>MANPTLFVSYDQNGKKLSFANWISVLSPQDTPFVSMTGKESINQTIFSWQTDALASVDGNNAHVEGSRAEDGEMKPTVIKSNVTQILRKVVRVSDTANTTANYGRGRELMYQLEKKGKEIKRDLEKILLSGQARTDVLADQYLTNSAADPAVAGLNDTHAARKTGAFQFLCAHGGLAGGVVDKTKNGPADPDTGAVTVKVAQNASNPTTNIGFDEADIFDMTLQLYTAGSEADIIMINPAHAKIFAGLQENTQGSRKRIFENTKQFIYEVNSITDPLGQSYKIIVNRWMPTDAVYFFRSADWTQMVLRAPKRTELAKDGSYEKWMIEMEVGLRHRNPYASGVLFTAAGKAAA[95x];>MAIETNAVVITDLNPLYPRDRDYIYEGAAQIRLIKQTLQNTFPNVTEPVDIDSDTFKIMSEKLKFTGDAMDVGGLMIKNVTPGTGDKDVVTKGQMEAFMKNWMENKLYRIGSYYITEEDINPGDSISLGFGSWAKVTGVIMGTGVVNPDGSVPNAQRVEFQAGGTGGRVFNTIRTENVPLMTVNGSSFSLSSNTHSHNMVFGRGDASGHNSSPNWYSPGGGYSQRTDNDTHTHTISGSVSLGRDDISRQPINTLPPFRAAHIWRRIS[3x];>[2x]MAMPDVQYPINTYGWLKKAVALWADRDDDEFVNQIPNFINFAEKEIYRNLRIPPLEKEVYLDIKDGVAYIPPDYLEAQWMMRAKDGTIFQVTSPEEISYRRQHGTINPSHWNNQPVNFARFGSRFIFYPSIEADTPYYPDDGSPLIPAENSVILSYYADPPEFHEDTDTSTILTIAPELLLYFTLRHACLFVQDDNGVQKWSALGKAILDEMVEQNKKQEYSGSPIAIPNNMTRLQSSLPDIYGIRTSRV;> MALYPIKSLGAVGVIADQAPTDLAPNAFTNAINARFVEQRVFKTGGNAPLSYVDEDKDLTPLSFVSMPFDYYSAGNSFLVVGTNKKLYKLTDESLTDISRKVATVTKKASASIKIYPVVSQIVPKESTISMNFNQTKNLEVSLLPADANNTNLIWEVSNSSYGSITVDPSDSKLATLTSFEKEGNLVVTISTANESVVAQIAVNIIDGDSGIFLSQDTVTIRKGGTTTLTAVTGKTPVTWSSNNASIVSVTPNANSLTAVITANGEGNVTITADNGTKTASCEIVSIPQIDSISLSQSDVTVSRGSQYILTATLSPANAPNQNITWTSSNPNIATVSGTSTQGTINALLAGFTEITATTEEGNRVAVCTVRVDLAGRTMRTSAMAFAAPVSESVETQEEEVVTPPESEETVYFAEPTSGIDTSGMYEGNNFYDYSNVNDIEGFARASLLATPLSSVTLDIVSASLDVGEEIVITATASPEGEYSYQWSVDKTGYVSTTSVTGKSIKLVALRKGEINVTCTVSQMTQKDYDAFDDYPWYHAVISNCAVATTHYETPQVKEFESEYFVDLPGWGEQTVVDNDGNPSVKKFNWKCERVRSFNNRLFALNMREANASGVTTNYPLRLRWSNFANENKAPTLWDDFAYDRVVSSDLASNIVGQTQALENGYAGYIDLADSNGSLIDILPLKDYLFVYTEFETYIGSPTNNTYQPLMFKKLFNDSGILAPECVVEVEGSHFVVTQNDVILHNGATKKSIASNRVKNMLINEVCLVNPLATRVHLHQDKKEVWVLYVGPGEPKESFACTKAAVWNYEFDTWSFRTIPYAQCIGLVDPPVLERGPIWSDFQEITWDDPSIKELVWRKDATNFRQRVTIVGSFLKGFYQVDVGALDYFYDRLNDVVIEKPLEMRLERTGIDFDNVTNEWNQKHINRFRPQTTGSGTYIFEAGGSQFSNEYGHPHTSKTYTIGVDRHVSVRLNHPYLFYNVIDNDVNSNAAINGLTIEFAVGGRR;>[3x]MIVYNNQAPDAVNNVGQFGATEGSIGAYKQAAEYAADSKYWALLAESKFGTIDDLIAEVERLYQQGVLMKQDIEDLKQDFKDQDARLMSLIAQTNAAVSDANNAVALINQKLIEVQNQLDVLLGMSVDVTTLPPGTPATGSFNPNTGVISLGIPEGEPGKDGSVKDLDTAPTGVPELGDLGFYVDKDDNTVHKTTLENIANLTPSVRSVSVNGGPALDGEVALTINKETVGLGNVLNVAQYSRQEINDKFDKTTKTYQSKAEAYADAQYRQVGEKVLVWEATKYEFYTVAANKTLTPVKTEGRILTVNSRSPDSSGNIDITIPTGNPSLYLGEMVMFPYDPSKNISYPGVLPADGRLVSKESASDLGPSLVSGQLPVVSETEWQSGAKQYFSWGKLADGITDADSTNFINIRLPDWTGGEAIRAPDSDKDSQYNGSVQAQKPYVVTVNNQAPDEITGNVNISRSILGAASSGANSDITSLSGLTTPLSISQGGTGAKDAASARSNLGLGSVSTLDNVPIASGGTGAGDAAGARFNLGLGNSATMNTGTNSDNVLKVGDFGIGRPDGALVFDTTSQDQLLAGLDTYGLCVFRNNQQIAAPWDIWNYSSNLFFRAGDTYSMISIPFESAGKIKVFGGASGSGWKTSRTVYDTVNTTVDVNGFIKAASPIVKVFHDGSFETNEQSDGVSVKKISTGVYLISGCLGLNSDAGWGGVDGGFEIPIDRNKQPRVWLDYEVKEDGSLLIKTYHRTHSTSPAFARNELEGFSDGDPVDIPKDAFISVRVEMPSK;>MGAGGFRKNTGRNNTTLPYNVGFLNNVQDTETYNVAVYDELQKVSTATNQMFQAIDEIHEEIDVRIKALNAMNLQFDELENRITTEIETAIADIQTQMGNLSTEDIWDNSVQPPVKLESTVSGFKTSIEGNTTKIQTVEGIVNDQGQEIALVQTELQNINGSLSQYMKLSEYEATWGVNSTVNGRYAGVKLTNNGTNSQFQVTANKFIVGDGSSGNTPFVFEGGRARMEFADIKNVNITTAQIANARIQWAQIDNVSISNAQIQNLSADKITAGSMWGSNWRLTVGGDFVMGGTGGAQLWMNGNRIDFYDGSGALRIRIGSW[3x];>[2x]MAKQKYSEEVLDELRVDLQRRFNYAQGYVDMAVKGYAREAWEYFYGNLPAPVTAGSSSWVDRTVWESVNGTLQDIINVFCSGDEAVTFVADNQQDSDAADVATKLVNQILLRDNPGYNIISSAAQECLVTRNSFIKYYWDEQTSTQTEEAEGVPPEALAAYVQGLEAGGLKNLEVFTEENEDGTVDVKVTYEQTVKRVKVEYVPSEQIFVDEHATSFAD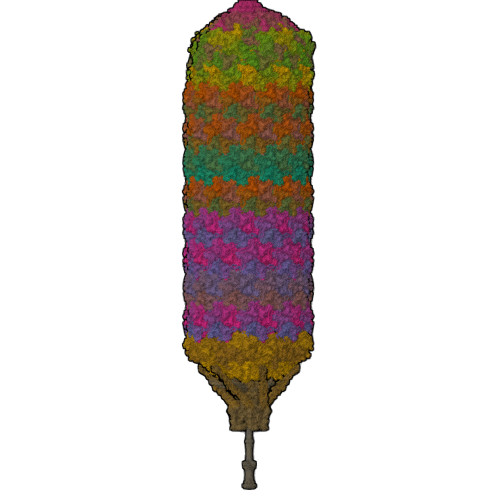AQYFCHRVRRSKEDLVAMGFPKDEIEAFNDWTDTMDTTQSTVAWSRTDWRQDIDADIGTDTEDIASMVWVYEHYIRTGVLDKNKESKLYQVIQAGEHILHTEEVTHIPFVTFCPYPIPGSFYGQSVYDITKDIQDLRTALVRGYIDNVNNANYGRYKALVGAYDRRSLLDNRPGGVVEMERQDAIDLFPYHNLPQGIDGLLGMSEELKETRTGVTKLGMGINPDVFKNDNAYATVGLMMNAAQNRLRMVCRNIAHNGMVELMRGIYNLIRENGEVPIEVQTPRGMIQVNPKQLPARHNLQVVVAISPNEKAERAQKLISLKQLIAADAQLAPLFGLEQDRYMTAQIFELMGIKDTHKYLLPLEQYQPPEPSPMEILQLEMTKAQVENVQASSQKMIADAFDQRERTTFEQQKAADELSLRQEELQFKQENAADAMTLENRKEDNNATLEQAKHKLALMQQQVRQYESVLKELQMVMSHQVDQEKIVQQARVQDKTLELQKKEANVTKKEQQASLKDSRIPGKRLGSKK7-{[3-({[(6-aminopyridin-2-yl)methyl]amino}methyl)phenoxy]methyl}quinolin-2-amine | C23 H23 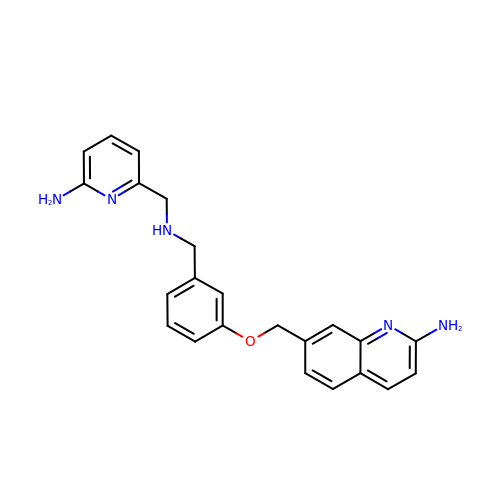N5 O | NZFRFODKYHOBEA-UHFFFAOYSA-N4-[(5-methoxypyridin-3-yl)sulfamoyl]benzene-1-sulfonic acid | C12 H12 N2 O6 S2 | 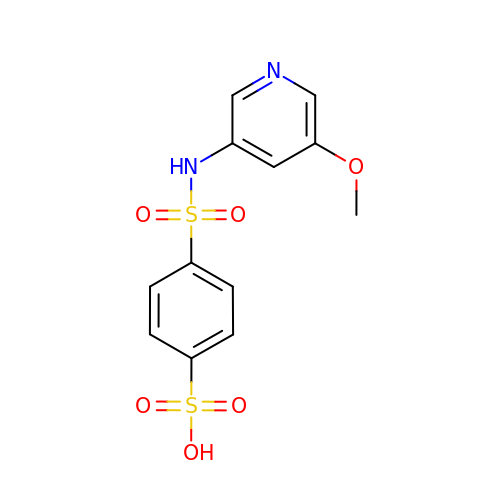PNZGKLKJTVFOSH-UHFFFAOYSA-N> MERLIPIVNKLQDLFAETGLDSPIDLPQIMVVGAQSSGKSSVLENVVGESIFPRGTGIVTRRPIVVQLYCTARERLNQSGAPDNMFNEDGSYVLSDGAPTDPRSIPPGAENQAYAEFLHKPGVRFYNFDDVRAEIERETDRVTGKNKGISPKAINLRVYSPHVVNLTVVDLPGLTKVPVGDQPSDIERLIRAMVLSYIERPNAIILAVHPATMDLATSDALQIARQADPEGRRTLGVITKLDLMDKGTDAMEMLTGKVIPLKLGYIGVICRGPADLRAGKSIQQAREDEIRFFRSHPVYRRLLPQLGTNTLARTLSTLLMKHIRDTLPSIRQKMSQQLAEWRKELQTLGPAFEGADDLGGALLNVINRYSSEFAKSLEGNSQQTVNTQELYGGARINYIFNDIYAKELQSMNAFEGLTREDIRTAIRNATGHRSPLFVPELAFELLVKKQITHFVPPAYSCVDLVYDELVRLALNCETELLQRYENLRSEILACAQNLLRELKQPCLEMVQNLIAMETSYISVNHKDFIGGNKAMSQLVRARMEEEERRTRSAKAANSTDNAANSAPKESNANDNRILQPRRRNQDE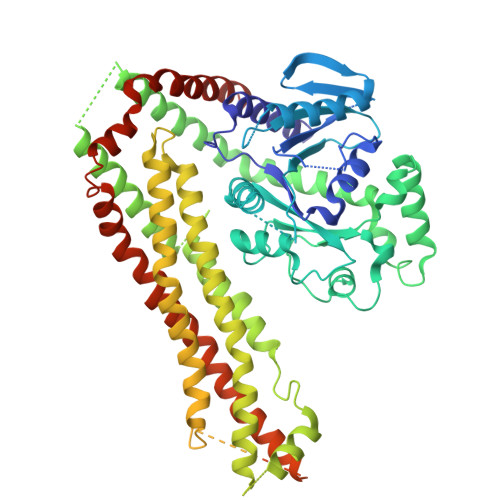NAKKNDDARRKDDKSPNKTDASNAEKDARSDRNPRGDPTMDNFFNEADEDEEDGNERRNRGLHTLPSVPEHLKAGEVSSDRDRDDIELIQTLLASYFDVVRVNMMDMVPKAIMSFLVLRARDRMQSRLVADLYKPERMSELLNESSDVAERRATAKRMVDLLQRGMAVINEVRDVHVKEEIHHHHHH methyl 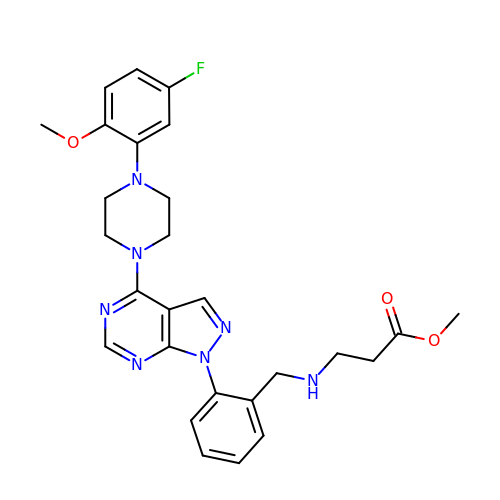N-[(2-{4-[4-(5-fluoro-2-methoxyphenyl)piperazin-1-yl]-1H-pyrazolo[3,4-d]pyrimidin-1-yl}phenyl)methyl]-beta-alaninate | C27 H30 F N7 O3 | PPQJOTCLVQMNEO-UHFFFAOYSA-N> LEEKKVCQGTSNKLTQLGTFEDHFLSLQRMFNNCEVVLGNLEITYVQRNYDLSFLKTIQEVAGYVLIALNTVERIPLENLQIIKGNMYYENSYALAVLSNYDANKTGLKELPMRNLQEILHGAVRFSNNPALCNVESIQWRDIVSSDFLSNMSMDFQNHLGSCQKCDPSCPNGSCWGAGEENCQKLTKIICAQQCSGRCRGKSPSDCCHNQCAAGCTGPRESDCLVCRKFRDEATCKDTCPPLMLYNPTTYQMDVNPEGKYSFGATCVKKCPRNYVVTDHGSCVRACGADSYEMEEDGVRKCKKCEGPCRKVCNGIGIGEFKDSLSINATNIKH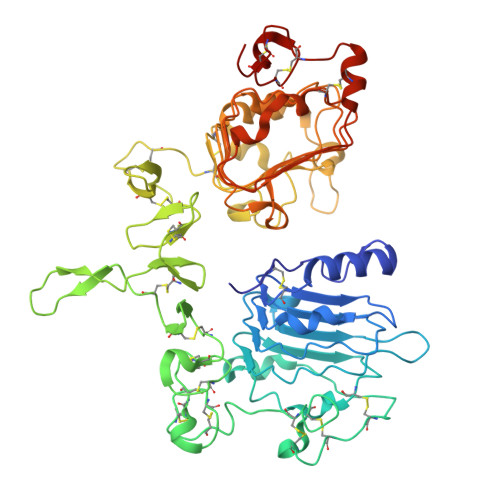FKNCTSISGDLHILPVAFRGDSFTHTPPLDPQELDILKTVKEITGFLLIQAWPENRTDLHAFENLEIIRGRTKQHGQFSLAVVSLNITSLGLRSLKEISDGDVIISGNKNLCYANTINWKKLFGTSGQKTKIISNRGENSCKATGQVCHALCSPEGCWGPEPRDCVSHHHHHH>[2x]SFGSDVRPAAAQEVVGGGDLGPNVLVFDPSTPDIQGKVDEVFRKQESNQFGTDRYALMFKPGTYNDINAQIGFYTSIAGLGLNPDDTTFNGDVTVDAGWFDGNATQNFWRSAENLALNPVNGTNRWAVSQAAPFRRMHVKGGLNLAPDGYGWASGGYIADSKIDGEVGPYSQQQWYTRDSSVGGWGN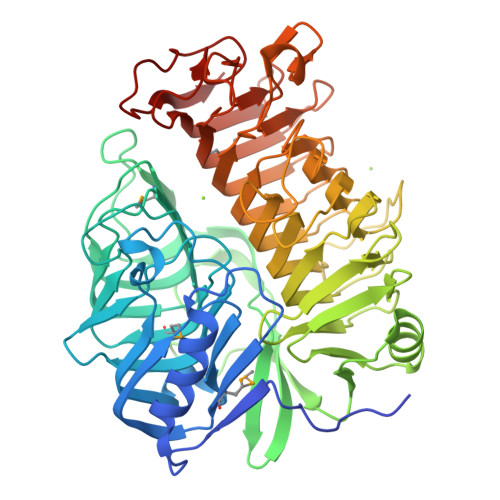GVWNMTFSGVEGAPAQSFPEPPYTTLETTPVSREKPFLYLDGDDYKVFVPAKRTNARGTSWGNGTPEGESLPLDQFYVVKPGATAETINAAVDQGLHLLFTPGVYHVDQPIEIDRANTVALGLGLATIIPDNGVTALKVGDVDGVKVAGLLVDAGPVNSETLVEVGSDGASGDHAANPTSLQDVFVRIGGAGPGKATTSIVVNSNDTIIDHTWVWRADHGEGVGWETNRADYGVHVKGDNVLATGLFVEHFNKYDVQWSGENGKTIFYQNEKAYDAPDQAAIQNGDIKGYAAYKVDDSVTTHEGWGMGSYCYFNVNPDIRQQHGFQAPVKPGVKFHDLLVVSLGGKGQYEHVINDIGDPTSGDTTIPSQVVSFP>MGTFIELVKNMKGY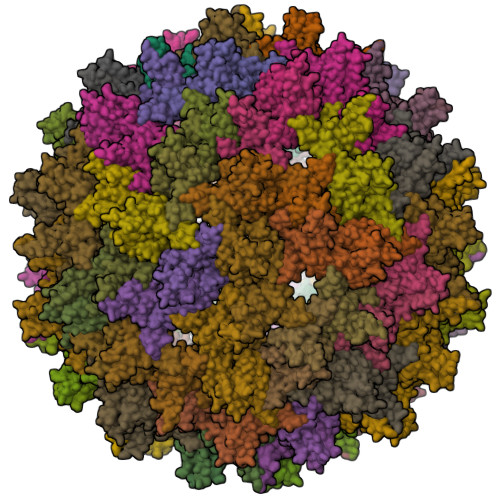KELLLPMEMVPLPAVVLKHVKLILTSQKEHQPWMTEMALKADQCLIHKATLDLAGKATSNEAKPLIEAMQQIILAMTRELWGQIQRHHYGIVQVEHYVKQITLWQDTPQAFRGDQPKPPSFRSDGPTRGQGSFRPFFRGRGRGRGRGRGSQSPARKGPLPK[180x]4-({4-[(2-cyanophenyl)amino]pyrimidin-2-yl}amino)benzoic 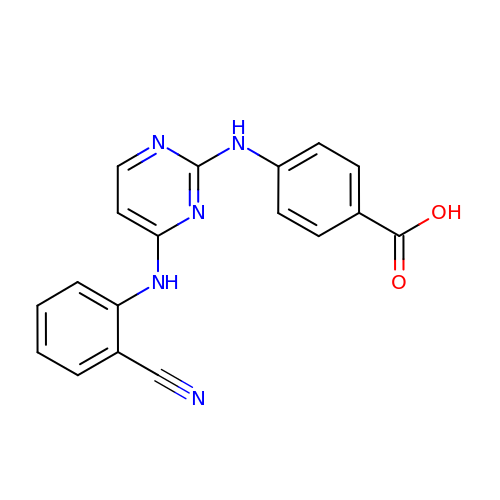acid | C18 H13 N5 O2 | MEKVNSMGVQRYJI-UHFFFAOYSA-N>MGHHHHHHGENLYFQGGSMAFPKKKLQGLVAATITPMTENGEINFSVIGQYVDYLVKEQGVKNIFVNGTTGEGLSLSVSERRQVAEEWVTKGKDKLDQVIIHVGALSLKESQELAQHAAEIGADGIAVIAPFFLKPWTKDILINFLKEVAAAAPALPFYYYHIPALTGVKIRAEELLDGILDKIPTFQGLKFSDTDLLDFGQCVDQNRQQQFAFLFGVDEQLLSALVMGATGAVGSTYNYLGKKTNQML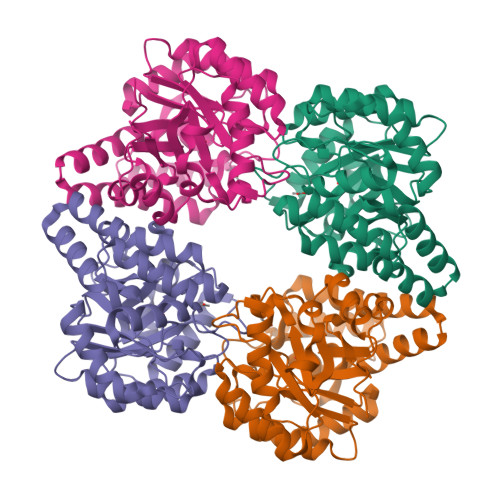EAFEQKDFSLALNYQFCIQRFINFVVKLGFGVSQTKAIMTLVSGIPMGPPRLPLQKASREFTDSAEAKLKSLDFLSFTDLKDGNLEAGS[4x]>[2x]MLITDTLSPQAFEEALRAKGDFYHIHHPYHIAMHNGNATREQIQGWVANRFYYQTTIPLKDAAIMANCPDAQTRRKWVQRILDHDGSHGEDGGIEAWLRLGEAVGLSRDDLLSERHVLPGVRFAVDAYLNFARRACWQEAACSSLTELFAPQIHQSRLDS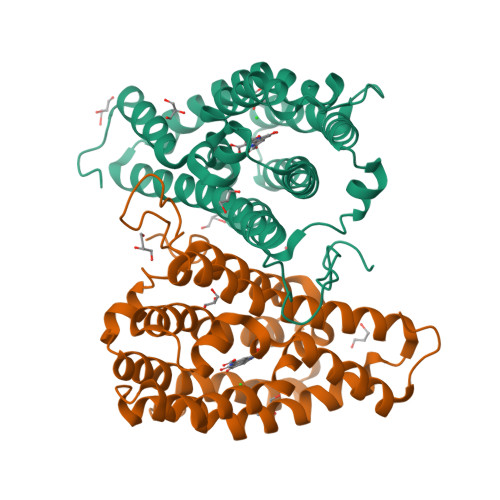WPQHYPWIKEEGYFFFRSRLSQANRDVEHGLALAKAYCDSAEKQNRMLEILQFKLDILWSMLDAMTMAYALQRPPYHTVTDKAAWHTTRLVLEHHHHH[(2S)-4-methyl-3-oxo-2,3,4,5-tetrahydro-1H-1,4-benzodiazepin-2-yl]acetic acid | C12 H14 N2 O3 | 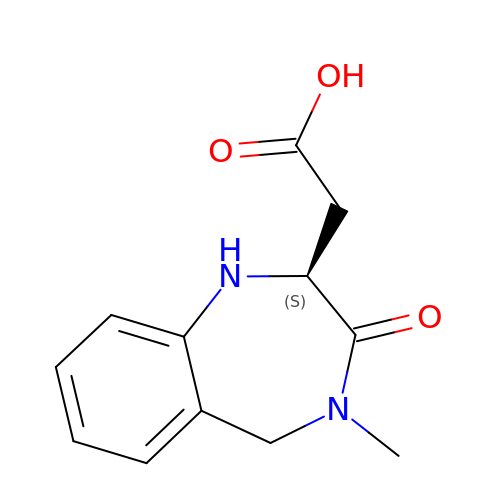CLWDLBDPVUWYEW-JTQLQIEISA-N> CCG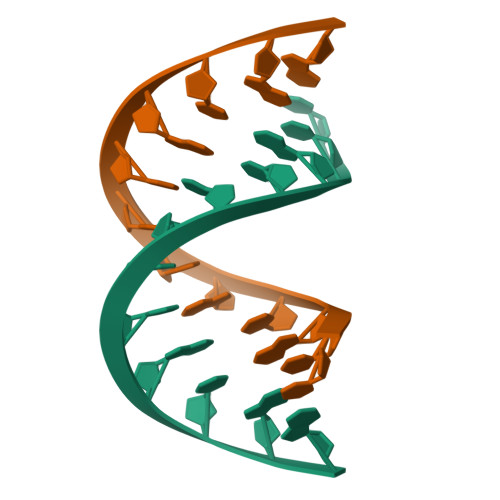TACGTACGG> MSSDVQAKLSGLLGDIGVKCTLAFAGTVAAGAAIVVPSGKQVEAASLDIY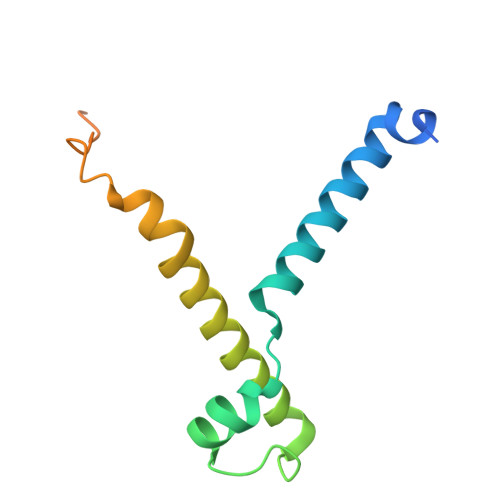GRPPSQLLPNERRAAEFAAGHRRWKGFVDNSIYSWTRTLPGHDNPIVNPYKGPRRPQRPQQKLEEEVEAAAKQE>AMSSMQFTDKATETLNAAAKYAAENSHVQLHPSHVAVVMLDEENSLFRSILEKAGGDVVSIERGFKKIMVRQPSQDPPPTEMGHSPELAKLLHYAHEHMKKQRDLYIAQDHLILALADLPSMAQVLKEGGVTKKSLENAVTHVRGNRRVESKSAEEAYEALSKYCIDLTELAASGKLDPVIGRDEIISRVIRVLSRRTKNNPCLVGEPGVGKTAIAEGLANRIVKGDIPSSLQKKVYSLDIGSLLAGAKYRGEFEERLKAVLKELKEAQAIVFIDEIHTVLGAGKSEGAIDAANLLKPMLARGELRCIGATTLTEYRQYVEKDPAFERRFQLVMVEEPSVTDTISILRGLKERYETHHGVRIADAAIVAAAQLAARYITQRFMPDKAIDLIDEACANTRVQLDSQPEAIDKLERRHLQLEVEATALEKEKDAASKQRLQEVRAEMARIQEELRPLKMKYESEKGRLDEIRNLSQRLDELKAKAEDAERRYDLARAADIRYYAIPDLEKRLAQLQAEKSQADAERADGLLAEVVGPDQIMEVVSRWTGIPVSNLQRSEKEKLLHMEEYMKQHVVGQDEAIKAICDAIRLSRTGLQNRNRPLASFLFLGPTGCGKTLCVKELAAFLFNDPG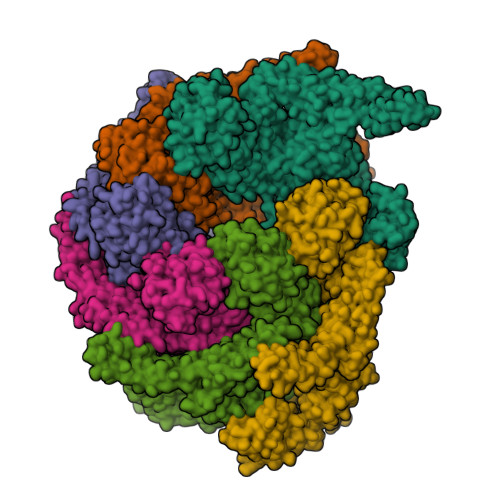AIVRIDMSEYMEKHAVSRLVGAPPGYIGHDEGGQLTEAVRRRPYTVVLFDEMEKAHKDVSNLLLQILDDGHCTDSKGRRVDFKNTIIVMTSNLGADLFELDEGDKVSQATKNAVLATARRHFANEFINRIDELIVFNRLTPSNIRKIVDVRLKEVQERLDEKQITLDVDDKAKDLLAQQGFDPVYGARPLNRLIQHALLTQLSRLLLDGGVRPGEIAKVTVDQEGEIIVIRNHGIESPAPWADEDMVEDEDMEI[6x]>SNAAIDVSAKSAIIIDGASGRVLYAKDEHQKRRIASITKIMTAVLAIESGKMDQTVTVSANAVRTEGSAIYLTEGQKVKLKDLVYGLMLRSGNDAAVAIAEHVGGSLDGFVYMMNQKAEQLGMKNTRFQNPHGLDDHENHYSTAYDMAILTKYAMKLKDYQKISGTKIYKAETMESVWKNKNKLLTMLYPYSTGGKTGYTKLAKRTLVSTASKDGIDLIAVTINDPNDWDDHMKMFNYVFEHYQTYLIAKKGDIPKLKGTFYESKAFIKRDITYLLTEEEKENVKINTTLLKPKKAWEK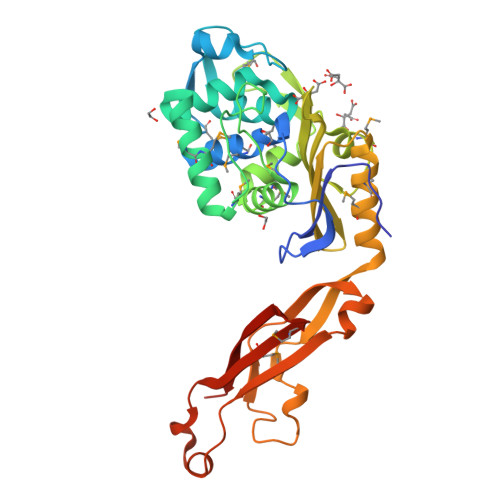DASKIPDIVGHMEIMFNDATIAKVPIYYENERHQK[2x]>[2x]GPLGSPHKCPDCDMAFVTSGELVRHRRYKHTHEKPFKCSMCDYASVEV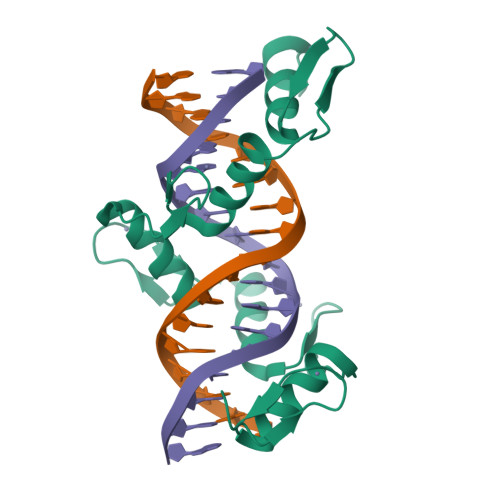SKLKRHIRSHTGERPFQCSLCSYASRDTYKLKRHMRTHSGEKPYECYICHARFTQSGTMKMHILQKHTENVAKFHCPHCDTVIARKSDLGVHLRKQHSYIEQ> MPAFDKPKVELHVHLDGSIKPETILYYGRRRGIALPANTAEGLLNVIGMDKPL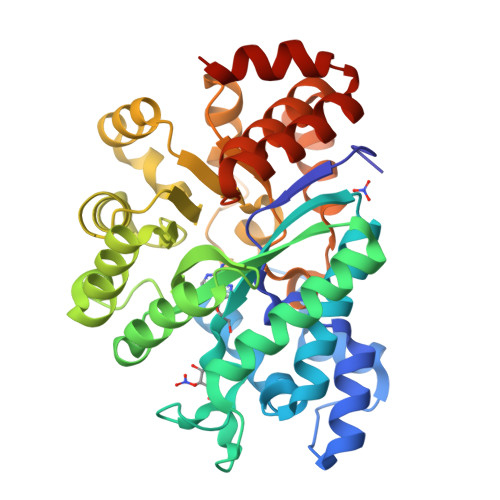TLPDFLAKFDYYMPAIAGCREAIKRIAYEFVEMKAKEGVVYVEVRYSPHLLANSKVEPIPWNQAEGDLTPDEVVALVGQGLQEGERDFGVKARSILCCMRHQPNWSPKVVELCKKYQQQTVVAIDLAGDETIPGSSLLPGHVQAYQEAVKSGIHRTVHAGEVGSAEVVKEAVDILKTERLGHGYHTLEDQALYNRLRQENMHFEICPWSSYLTGAWKPDTEHAVIRLKNDQANYSLNTDDPLIFKSTLDTDYQMTKRDMGFTEEEFKRLNINAAKSSFLPEDEKRELLDLLYKAYGMPPSASAGQNLAENLYFQ>[6x]MKLPIHFYKPLAAGAPQPIRELPVRPERVIHFFPPHVEKIRAR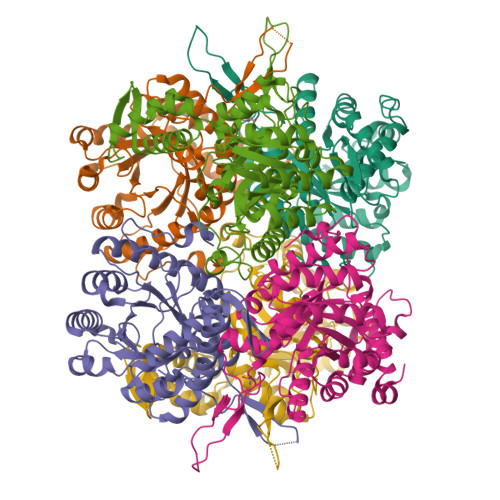IPEVAKQVDVLCGNLEDAIPIDAKEAARAGFIEVARNTDFGDTALWVRVNALNSPWVLDDIADIVATVGNKLDVMMIPKVEGPWDIHFVDQYLALLEAKHQIQKPILIHALLETAQGMMNLEAIAGASPRMHGFSLGPADLAASRGMKTTRVGGGHPFYGVLADPQEGQEHRPFYQQDLWHYTIARMVDVAVAHGLRAFYGPFGDIKDEAACEAQFRNAFLLGCTGAWSLAPNQIPIAKRVFSPDVNEVLFAKRILDAMPDGSGVAMIDGKMQDDATWKQAKVIVDLARMIAKKDPELAQAYGF>[3x]MSKLQISNTCPDKYRTKQEGVEYPTAKKITYYSKVTETERKMNVILPVGYDENKKYPVVYYLHGLMSYEDSMLEDDSTLAIPTNLLKEGRAKEMIIVLPDVYAPKPGTAVTPDFNPEYYKGYDNFINELIEVIMPYMEE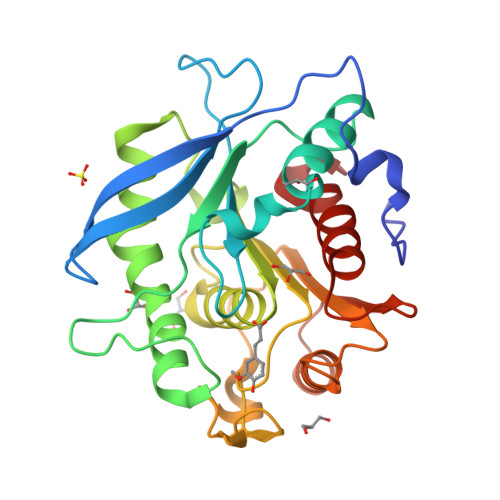HYSILTGRENTALCGFSMGARTSLYIGYMRSDLIGYVGAFAPAPGITPGEDSFSGKHEGLISEDEFRAEIQPIVSLIDCGTNDSVVGQFPKSYHEILTRNNQEHIWFEVPGADHDWNAISAGFYNFIQTTFGALNN> MPEITESERAYHLRKMKTRMQRVDVTGDGFISREDYELIAVRIAKIAKLSAEKAEETRQEFLRVADQLGLAPGVRISVEEAAVNATDSLLKMKGEEKAMAVIQSLIMYDCIDTDKDGYVS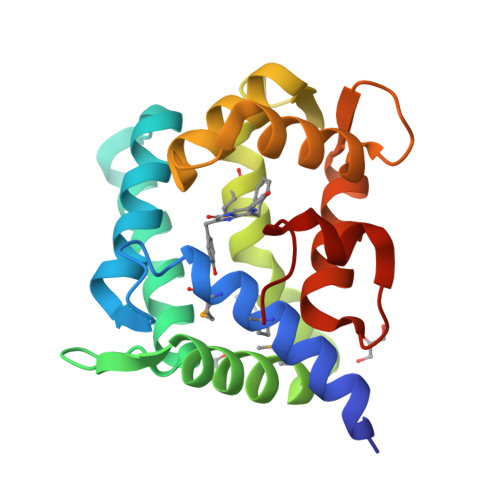LPEFKAFLQAVGPDLTDDKAITCFNTLDFNKNGQISRDEFLVTVNDFLFGLEETALANAFYGDLVD The heterotrimeric [FeFe] hydrogenase, HydABC, from T. maritima is a soluble cytoplasmic enzyme involved in fermentation. It uses electrons from the one-electron carrier ferredoxin (E°′ ≈ −450 mV Schut and Adams, 2009), which is reduced during pyruvate metabolism, and the two-electron carrier NADH (E°′ ≈ −20 mV; Schut and Adams, 2009), produced during glucose metabolism, to reduce protons to hydrogen (E°′ ≈ −420 mV; Schut and Adams, 2009). The electron-bifurcating [FeFe] hydrogenase from Thermotoga maritima (HydABC) requires both NADH and ferredoxin to reduce protons generating hydrogen. Electron bifurcation is a fundamental energy conservation mechanism in nature in which two electrons from an intermediate-potential electron donor are split so that one is sent along a high-potential pathway to a high-potential acceptor and the other is sent along a low-potential pathway to a low-potential acceptor.

To investigate the blurred regions, symmetry expansion followed by classification was explored to separate the different conformations into classes. Initial attempts to use D2 symmetry, to match the core, resulted in maps no better than before, however, using C2 symmetry revealed two classes with bridging density between the HydB lobes with local resolution similar to the lobes formed from HydA and HydB. This bridging density breaks the rotational symmetry between the protomers in the Hyd(ABC)2 unit, explaining why D2 symmetry expansion was ineffective. The two classes correspond to the bridge domain being formed between different HydB lobes: when rotated by 180°, the bridges are identical. Despite extensive attempts, we were unable to find a class with both bridges in the closed conformation. The observation that both bridges cannot close simultaneously suggests that these behave as reciprocating elements. In the bridge-containing structure, the two C-terminal [4Fe–4S] clusters (named B3 and B4) of HydB are close enough to exchange electrons with each other but are too far from the next nearest FeS clusters, such as cluster C1 (≈35 Å away) or cluster A5 (≈32 Å away). Furthermore, cluster A5 is completely isolated from exchanging electrons with all the nearest clusters being >30 Å away. Thus, unless the HydA and HydB bridge domains undergo substantial conformational changes, the FeS clusters A5, B3, and B4 cannot participate in electronic exchange with the rest of the enzyme. Fourier shell correlation (FSC) curves showing the resolution of (A, B) the ‘bridge closed’ maps, both reaching a resolution of 2.8 Å and (C), the ‘bridge open’ map, reaching a resolution of 2.7 Å (although note that the bridge is much less well resolved than the core in this particular map).

>[2x]MKIYVDGREVIINDNERNLLEALKNVGIEIPNLCYLSEASIYGACRMCLVEINGQITTSCTLKPYEGMKVKTNTPEIYEMRRNILELILATHNRDCTTCDRNGSCKLQKYAEDFGIRKIRFEALKKEHVRDESAPVVRDTSKCILCGDCVRVCEEIQGVGVIEFAKRGFESVVTTAFDTPLIETECVLCGQCVAYCPTGALSIRNDIDKLIEALESDKIVIGMIAPAVRAAIQEEFGIDEDVAMAEKLVSFLKTIGFDKVFDVSFGADLVAYEEAHEFYERLKKGERLPQFTSCCPAWVKHAEHTYPQYLQNLSSVKSPQQALGTVIKKIYARKLGVPEEKIFLVSFMPCTAKKFEAEREEHEGIVDIVLTTRELAQLIKMSRIDINRVEPQPFDRPYGVSSQAGLGFGKAGGVFSCVLSVLNEEIGIEKVDVKSPEDGIRVAEVTLKDGTSFKGAVIYGLGKVKKFLEERKDVEIIEVMACNYGCVGGGGQPYPNDSRIREHRAKVLRDTMGIKSLLTPVENLFLMKLYEEDLKDEHTRHEILHTTYRPRRRYPEKDVEILPVPNGEKRTVKVCLGTSCYTKGSYEILKKLVDYVKENDMEGKIEVLGTFCVENCGASPNVIVDDKIIGGATFEKVLEELSKNG;>MFKNAKEFVQYANKLKTLREKKLNGVSIYVCVGTGCTAKGALKVYSAFEEELKKRNLLGQVTLEKIDDDKVTLNRTGCCGRCSSGPLVKIMPYRFFYSNVAPEDVPEIVDRTVLKGEPIERLFLTDPLTGEKVPRIEDTTLFKNQDFYIMEAIGESECDSIEDYIARSGYESLVKALTSMTPEEIIETVKASGLRGRGGGGFPTGLKWEFTRKAQGDIKFVVCNGDEGDPGAFMNRTLLERDPHLVLEGMIIAGYAVGAQKGYAYIRAEYPFAVKMFKKAIEDARKLGLLGENILGTGFSFDLEVKEGAGAFVCGEETALLASIEGKRGMPRPKPPFPAQSGLWGKPTLINNVETYANIPRILRDGVENYRKRGTENSPGTKMFSVAGPLKATGIIEVEFGTTLRDIIYNICGGFVEGEEFKAVQIGGPSGACLSEDFIDMPLDYDTLKKADAMVGSGGIVVITKKTCMVEVARFFLDFTKRESCGKCVPCREGTMQAYNILEKFTHGKATYEDLKTLEHLSKTIKTASLCGLGKTAPNPILSTLKLFREEYIAHIEGECPSGMCTAFKKYVINPDICKGCGLCARSCPQNAITGERGKPYTIDQEKCVKCGLCASKCPFKAIELV[2x];>[2x]MASWSHPQFEKSGGGGGENLYFQGAVLALERHFEKVEEILKKYGYKRENLIKILLEIQEIYRYLPEDVINYVSTAMGIPPAKIYGVATFYAQFSLKPKGKYTIMVCDGTACHMAGSPEVLKAIEEETGLTPGNVTEDLMFSLDQVGCLGACALAPVMVINGEVYGNLTADKVKEILRKIKEKERESANV> LEEKKVCQGTSNKLTQLGTFEDHFLSLQRMFNNCEVVLGNLEITYVQRNYDLSFLKTIQEVAGYVLIALNTVERIPLENLQIIRGNMYYENSYALAVLSNYDANKTGLKELPMRNLQEILHGAVRFSNNPALCNVESIQWRD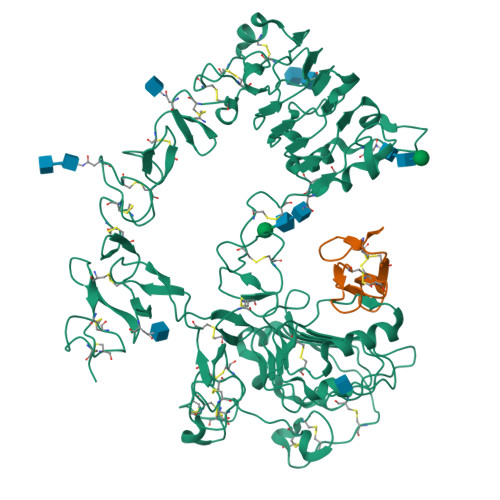IVSSDFLSNMSMDFQNHLGSCQKCDPSCPNGSCWGAGEENCQKLTKIICAQQCSGRCRGKSPSDCCHNQCAAGCTGPRESDCLVCRKFRDEATCKDTCPPLMLYNPTTYQMDVNPEGKYSFGATCVKKCPRNYVVTDHGSCVRACGADSYEMEEDGVRKCKKCEGPCRKVCNGIGIGEFKDSLSINATNIKHFKNCTSISGDLHILPVAFRGDSFTHTPPLDPQELDILKTVKEITGFLLIQAWPENRTDLHAFENLEIIRGRTKQHGQFSLAVVSLNITSLGLRSLKEISDGDVIISGNKNLCYANTINWKKLFGTSGQKTKIISNRGENSCKATGQVCHALCSPEGCWGPEPRDCVSCRNVSRGRECVDKCKLLEGEPREFVENSECIQCHPECLPQAMNITCTGRGPDNCIQCAHYIDGPHCVKTCPAGVMGENNTLVWKYADAGHVCHLCHPNCTYGCTGPGLEGCPTNGPKHHHHHH;> NSDSECPLSHDGYCLHDGVCMYIEALDKYACNCVVGYIGERCQYRDLKWWELR> HPETLVKVKDAEDQLGARVGYIELDLNSGKILESFRPEERFPMISTFKVLLCGAVLSRVDAGQEQLGRRIHYSQNDLVEYSPVTEKHLTDGMTVRELCSAAITMSDNTAANLLLTTIGGPKELTAFLHNMGDHVTRLDRWEPELNEAIPNDERDTTTPAAMATTLRKLLTGELLTLASRQQLIDWMEADKVAGPLLRS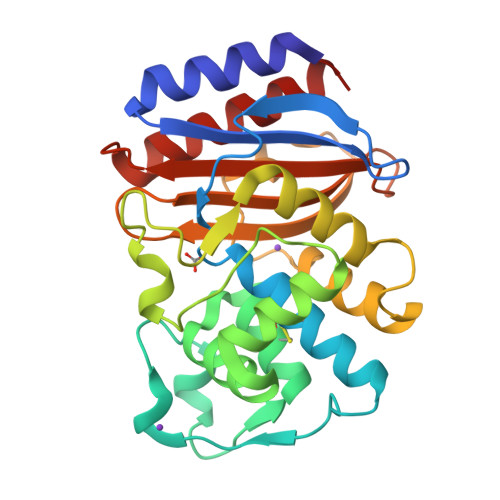ALPAGWFIADKSGAGERGSRGIIAALGPDGKPSRIVVIYTTGSQATMDERNRQIAEIGASLIKHW> METPLDLLKLNLDERVYIKLRGARTLVGTLQAFDSHSNIVLSDAVETIYQLNNEELSESERRSEMVFIRGDTVTLISTPSEDDD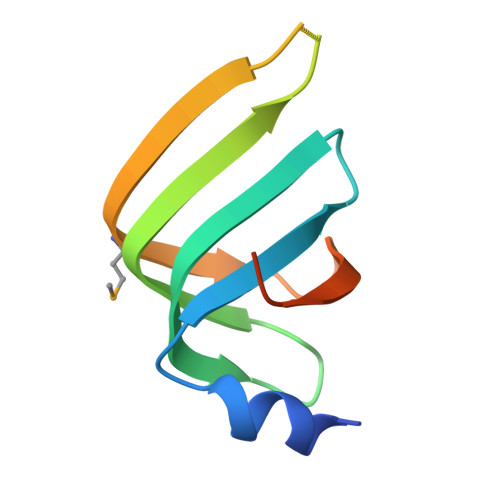GAVEI>MS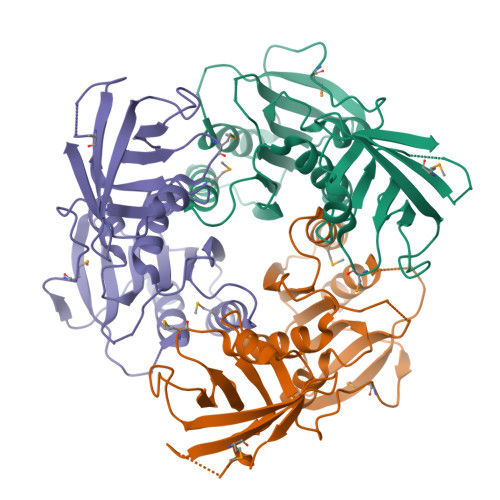LGIYMRDDILDIITLTTDFGTNEGYVGAMKGRILNILKKYNKDAKIIDISHEIKPFNIYHGAYVLLTAIPYFPPSVHVAVIDPTVGSERKSIVIETKSGYYLVGPDNGLFTYVAEKLGIKRIIKIDEERYKPSSTFHGRDVYAVVGAEILINNGYDGEELDEMVKIDETKKRVIHIDRFGNIITNIKKDEVTFKYYDTIMIKIRHKNGIEKIIKCKFVKSYFEEKNNFICLINSEGFLEISKFMDNASKLLNVDYLDEIEIEGGSHHHHHH[3x]>MAVLSSADRASNEKKVKSSYFDLPPMEMSVAFPQATPASTFPPCTSDYYHFNDLLTPEEQAIRKKVRECMEKEVAPIMTEYWEKAEFPFHITPKLGAMGVAGGSIKGYGCPGLSITANAIATAEIARVDASCSTFILVHSSLGMLTIALCGSEAQKEKYLPSLAQLNTVACWALTEPDNGSDASGLGTTATKVEGGWKINGQKRWIGNSTFADLLIIFARNTTTNQINGFIVKKDAPGLKATKIPNKIGLRMVQNGDILLQNVFVPDEDRLPGVNSFQDTSKVLAVSRVMVAWQPIGISMGIYDMCHRYLKERKQFGAPLAAFQLNQQKLVQMLGNVQAMFLMGWRLCKLYETGQMTPGQASLGKAWISSKARETASLGRELLGGNGILADFLVAKAFCDLEPIY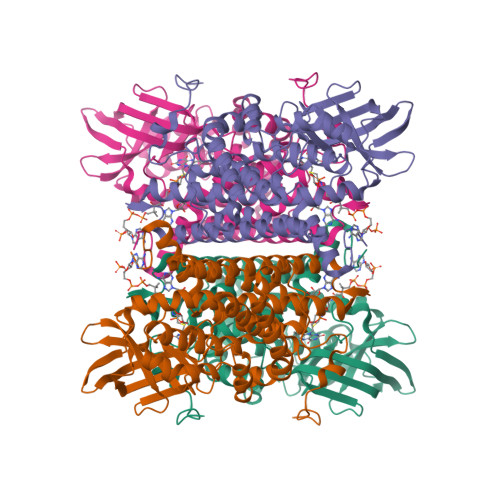TYEGTYDINTLVTGREVTGIASFKPATRSRL[4x]>SKLLKESFEGDGYHKGPKQVVALKATKLFTYDSIKSKKMFHATVATDTEFFRVMVFEENLEKKFIPGNTIALSDYFGMYGSLAIHEYSSVSEVKSQNKEDSSSSDERPIEHLKICDLHLQTEERLVDGEF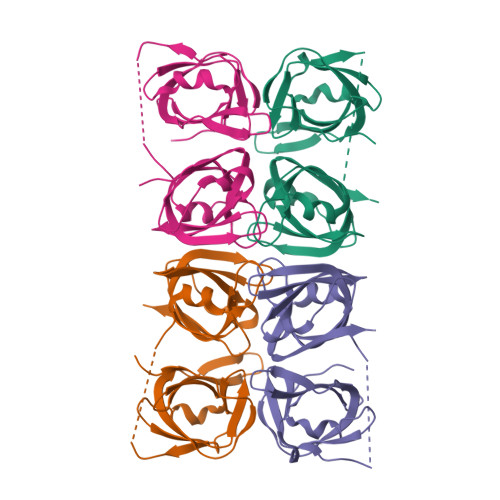KVYRKSSGNNCICYGIWDDTGAMKVVVSGQLTSVNCEIGNTIRLVCFELTSNADEWFLRATRYSYMEVIMPEK[4x]>[2x]GPAMLTTRIIKETEKLQKECPPGITATPTKENPRYFMVTIQGPPQSCYEGGLFRLELFLPEEYPMKPPKVRFLTRIYHPNVDKVGRICLDIIKDKWSPALLINKVLLSIQILMSSPNPDDPLANDVAEHWKEDEASALQTAREWTRKYAKP;>GPAMVEVPRNFRLLEELETGEKGTGSNQNVSVGLRDTADIFFHYWNGTIVGPPSTTFEYRILSLEIYCDENYPKVPPH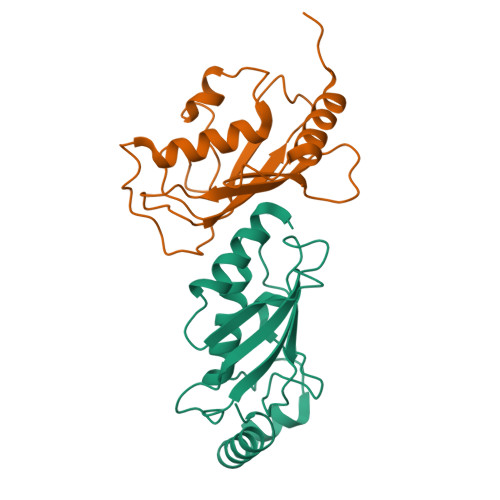IRFLSKVNLPCVDSDGTVNREKFHVFKHWDRRTTMELCLSELRKEMAQPQNRKLVQPPEGSTY[2x]> MGSSHHHHHHHHLEVLFQGPHMEWIQSLPKIELHAHLNGSIRDSTLLELARVLGEKGVIVFADVEHVIQKNDRSLVEVFKLFDLIHKLTTDHKTVTRITREVVEDFALENVVYLELRTTPKRSDSIGMSKRSYMEAVIQGLRSVSEVDIDFVTASDSQKLHNAGDGIGRKKIYVRLLLSIDRRETTESAMETVKLALEMRDVGVVGIDLSGNPLVGEWSTFLPALQYAKDNDLHITLHCGEVPNPKEIQAMLDFKPHRIGHACFFKDEDWTKLKSFRIPVEICLTSNIVTKSISSIDIHHFADLYN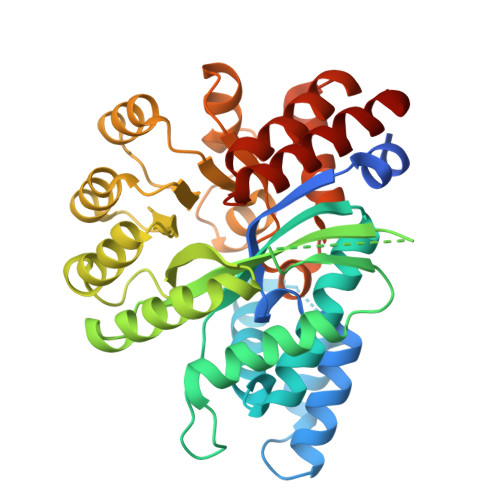AKHPLILCTDDFGVFSTSLSNEYALAVRSLGLSKSETFALARAAIDATFAEDEVKQQLRFIFDSASPEHV> IPLKGLLSIILRSHRVFIGRELGHLNLTDAQVACLLRIHREPGIKQDELATFFHVDKGTIARTLRRLEESGFIEREQDPENRRRYILEVTRRGEE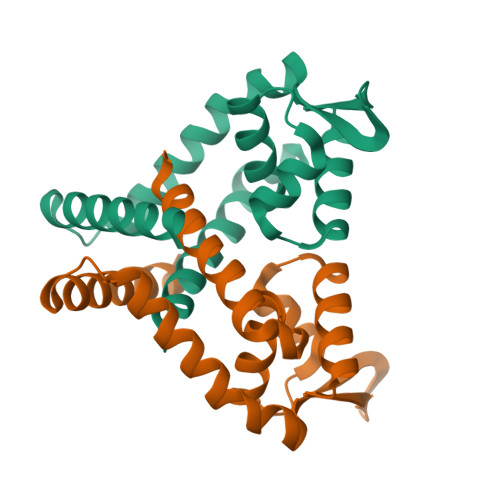IIPLILKVEERWEDLLFRDFTEDERKLFRKMCRRLAEEAVRMR>MRILVTNDDGIYSPGLWALAEAASQFGEVFVAAPDTEQSAAGHAITIAHPVRAYPHPSPLHAPHFPAYRVRGTPADCVALGLHLFGPVDLVLSGVNLGSNLGHEIWHSGTVAAAKQGYLFGLSAAAFSVPLNGEVPDFAGLRPWLLR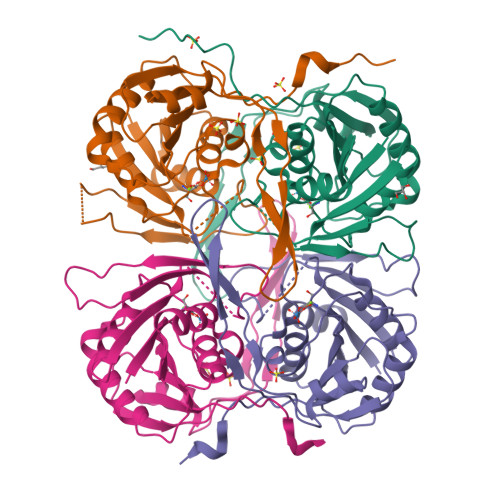TLETLLRLERPFLVNVNLPLRPKGFLWTRQSVRAYEGVVIPGEDPMGRPFYWFAPRPLKEAEEGTDRWAVAQGFVSATPLRLDLTDETRLQPTLAHD[4x]(2S)-5,7-dihydroxy-9-methyl-2-(prop-1-en-2-yl)-1,2,3,4-tetrahydro-6H-benzo[7]annulen-6-one | C15 H18 O3 | 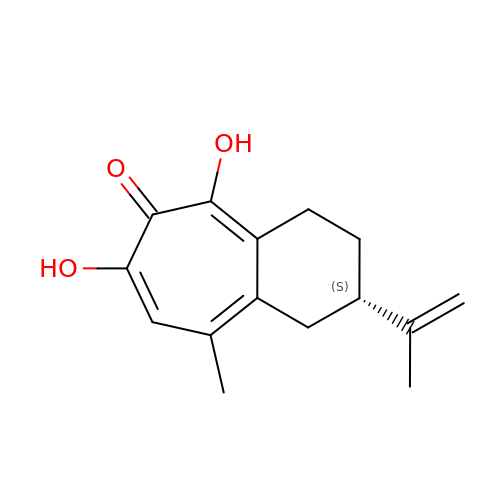XZCVMNQLRNHDOD-JTQLQIEISA-N> QKTRPFTVPNIPLKYLSNSRIPNPIEGMSLSPDQTQNVQFQNGRCTIDGQPLGTTPVSVSQLCKFRGRITSGQRVLNLTELDGSPFMAFAAPAPAGFPDLGSCDWHIEMSKIP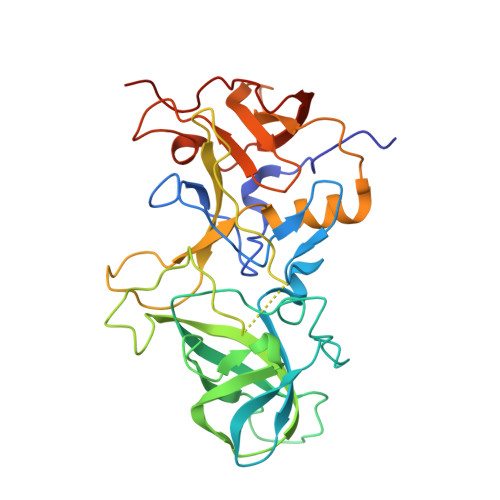NSSTQNNPIVTNSVKPNSQQFVPHLSSITLDENVSSGGDYIGTIQWTSPPSDSGGANTNFWKIPDYGSSLAEASQLAPAVYPPGFNEVIVYFMASIPGPNQSGSPNLVPCLLPQEYITHFISEQAPIQGEAALLHYVDPDTNRNLGEFKLYPGGYLTCVPNSSSTGPQQLPLDGVFVFASWVSRFYQLKPVGTAGPARGRL> MAMHPRKDWYELTRATNWTPSYVTEEQLFPERMSGHMGIPLEKWESYDEPYKTSYPEYVSIQREKDAGAYSVKAALERAKIYENSDPGWISTLKSHYGAIAVGEYAAVTGEGRMARFSKAPGNRNMATFGMMDELRHGQLQLFFPHEYCKKDRQFDWAWRAYHSNEWAAIAAKHFFDDIITGRDAISVA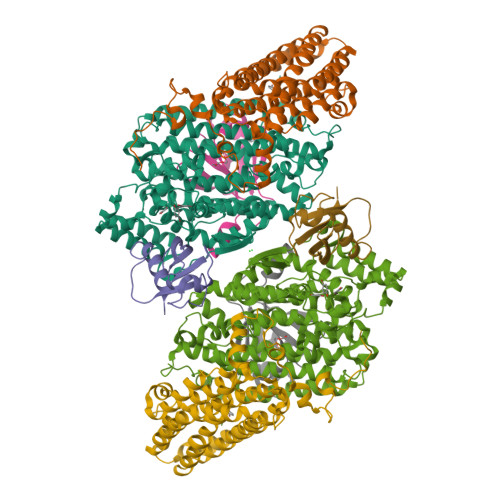IMLTFSFETGFTNMQFLGLAADAAEAGDYTFANLISSIQTDESRHAQQGGPALQLLIENGKREEAQKKVDMAIWRAWRLFAVLTGPVMDYYTPLEDRSQSFKEFMYEWIIGQFERSLIDLGLDKPWYWDLFLKDIDELHHSYHMGVWYWRTTAWWNPAAGVTPEERDWLEEKYPGWNKRWGRCWDVITENVLNDRMDLVSPETLPSVCNMSQIPLVGVPGDDWNIEVFSLEHNGRLYHFGSEVDRWVFQQDPVQYQNHMNIVDRFLAGQIQPMTLEGALKYMGFQSIEEMGKDAHDFAWADKCKPAMKKSA;> MSFESKKPMRTWSHLAEMRKKPSEYDIVSRKLHYSTNNPDSPWELSPDSPMNLWYKQYRNASPLKHDNWDAFTDPDQLVYRTYNLMQDGQESYVQSLFDQFNEREHDQMVREGWEHTMARCYSPLRYLFHCLQMSSAYVQQMAPASTISNCCILQTADSLRWLTHTAYRTHELSLTYPDAGLGEHERELWEKEPGWQGLRELMEKQLTAFDWGEAFVSLNLVVKPMIVESIFKPLQQQAWENNDTLLPLLIDSQLKDAERHSRWSKALVKHALENPDNHAVIEGWIEKWRPLADRAAEAYLSMLSSDILPAQYLERSTSLRASILTV;> MSAFPVHAAFEKDFLVQLVVVDLNDSMDQVAEKVAYHCVNRRVAPREGVMRVRKHRSTELFPRDMTIAESGLNPTEVIDVVFEE;> MSTLADQALHNNNVGPIIRAGDLVEPVIETAEIDNPGKEITVEDRRAYVRIAAEGELILTRKTLEEQLGRPFNMQELEINLASFAGQIQADEDQIRFYFDKTM Type 1 pili are important virulence factors of uropathogenic Escherichia coli that mediate bacterial attachment to epithelial cells in the urinary tract. The pilus rod is comprised of thousands of copies of the main structural subunit FimA and is assembled in vivo by the assembly platform FimD. The pilus rod is a right-handed superhelical structure composed of ~3.2 subunits per turn with an axial rise between two consecutive subunits of 7.8 Å or 7.7 Å for the type 1 and P pilus rods, respectively. All subunits in the rod are connected via DSE, forming an exceptionally stable fold that is resistant to extreme temperatures, denaturants and mechanical stress.

Our structures of in vivo-assembled, in vitro-assembled and FimD-cat pilus rods were resolved to 2.85, 2.69 and 2.52 Å, respectively. We modelled six adjacent FimA subunits linked through donor-strand interactions and refined the models against their respective cryo-EM maps. The Cα root mean square deviation (RMSD) from global alignment of the three models was less than 1 Å in each case (0.68 Å, 0.69 Å and 0.25 Å for FimD-cat vs. in vivo, FimD-cat vs. in vitro and in vitro vs. in vivo, respectively) implying that all three structures are highly similar. Indeed, the solid-state NMR spectra revealed structural differences between in vivo- and in vitro-assembled samples, where the resonance positions of a few residues exhibited small shifts, peak splitting and/or line broadening. Our experiments suggest that these structural differences occurred in approximately every third FimA subunit of in vitro-assembled pili, and that this could explain the observed stability difference. Additionally, we observed peak doubling and/or line broadening for a subset of FimA residues (V17, V23, V37, A69, A72, A93, I103, T128, F154 and Q159) in the in vitro sample. By contrast, pili assembled in vitro, without prior incubation with GdmCl, produced SEC profiles consisting of a void volume peak, a broad shoulder containing smaller pilus fragments of different lengths, and a peak of the unfolded FimA monomer. Following incubation with 4.1 M GdmCl, the smaller fragments became even more abundant, and after incubation with 6 M GdmCl, the pili had almost fully dissociated and unfolded. Taken together, these results suggest that when pili were assembled in vitro from FimA monomers or FimA–FimC complexes in the absence of FimD, structural defects occurred in the resulting pilus rods, likely at the positions where small fragments associated to longer fragments. When such in vitro-assembled pilus rod samples are subjected to medium to high GdmCl concentrations, rapid fragmentation occurs at the sites of quaternary structural defects, followed by the rapid dissociation/unfolding of the resulting small fragments.

>MKIKTLAIVVLSALSLSSTAALAAATTVNGGTVHFKGEVVNAACAVDAGSVDQTVQLGQVRTASLAQEGATSSAVGFNIQLNDCDTNVASKAAVAFLGTAIDAGHTNVLALQSSAAGSATNVGVQILDRTGAALTLDGATFSSETTLNNGTNTIPFQARYFATGAATPGAANADATFKVQYQ[6x]>[8x]GSHMGFLSGKRILVTGVASKLSIAYGIAQAMHRE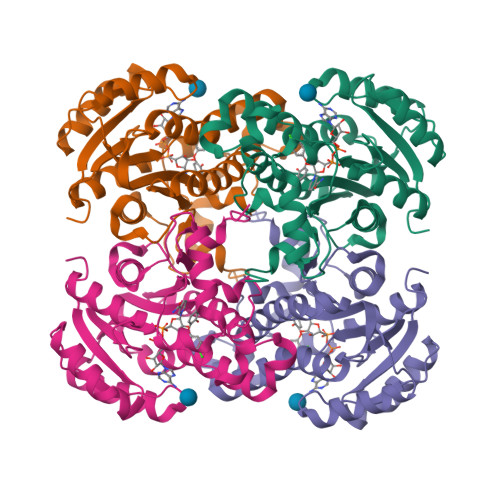GAELAFTYQNDKLKGRVEEFAAQLGSDIVLQCDVAEDASIDTMFAELGKVWPKFDGFVHSIGFAPGDQLDGDYVNAVTREGFKIAHDISSYSFVAMAKACRSMLNPGSALLTLSYLGAERAIPNYNVMGLAKASLEANVRYMANAMGPEGVRVNAISAGPIRTLAASGIKDFRKMLAHCEAVTPIRRTVTIEDVGNSAAFLCSDLSAGISGEVVHVDGGFSIAAMNELELK>[2x]GSHMGR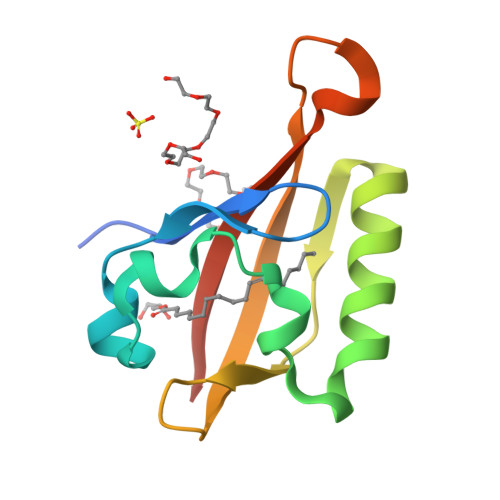GAFLSRHSLDMKFTYCDDRIAEVAGYSPDDLIGCSAYEYIHALDSDAVSKSIHTLLSKGQAVTGQYRFLARSGGYLWTQTQATVVSGGRGPQSESIVCVHFLISQVEET> CQPIFLNVLEAIEPGVVCAGHDNNQPDSFAALLSSLNELGERQLVHVVKWAKALPGFRNLHVDD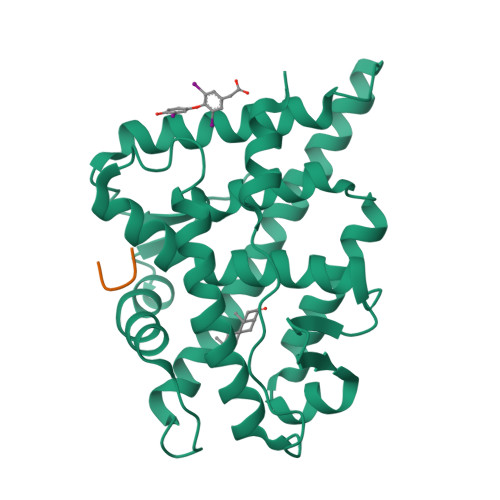QMAVIQYSWMGLMVFAMGWRSFTNVNSRMLYFAPDLVFNEYRMHKSRMYSQCVRMRHLSQEFGWLQITPQEFLCMKALLLFSIIPVDGLKNQKFFDELRMNYIKELDRIIACKRKNPTSCSRRFYQLTKLLDSVQPIARELHQFTFDLLIKSHMVSVDFPEMMAEIISVQVPKILSGKVKPIYFHTQ;> KLLF> MGSQPTNSHFTLNEQTLCGTNISLLGNNRFIQIGNGLHMTYAPGFFGNWSRDLTIGPRFGGLNKQPIHVPPKRTETASIQVTPRSIVINRMNNIQINPTSIGNPQVTIRLPLNNFKSTTQLIQQVSLTDFFRPDIEHAGSIVLILRHPSDMIGEANTLTQAGRDPDVLLEGLRNLFNACTAPWTVGEGGGLRAYVTSLSFIAACRAEEYTDKQAADANRTAIVSAYGCSRMETRLIRFSECLRAMVQCHVFPH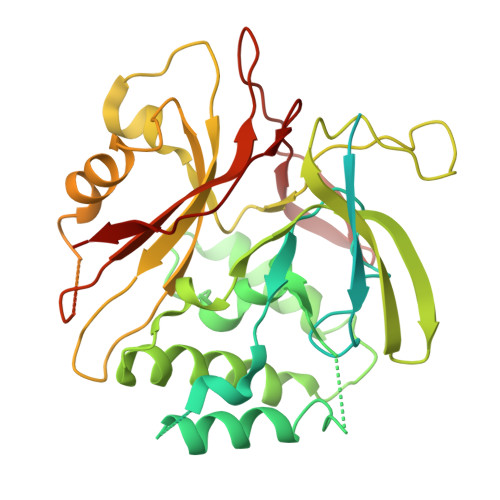RFISFFGSLLEYTIQDNLCNITAVAKGPQEAARTDKTSTRRVTANIPACVFWDVDKDLHLSADGLKHVFLVFVYTQRRQREGVRLHLALSQLNEQCFGRGIGFLLGRIRAENAAWGTEGVANTHQPYNTRALPLVQLSNDPTSPRCSIGEITGVNWNLARQRLYQWTGDFRGLPTQLSCMYAAYTLIGTIPSESVRYTRRMERFGGYNVPTIWLEGVVWGGTNTWNECYY> GAMEGFKANLSLLRRPGEKTYTQRCRLFVGNLPADITEDEFKRLFAKYGEPGEVFINKGKGFGFIKLESRALAEIAKAELDDTPMRGRQLRVRFATHAAALSVRNLSPYVSNELLEE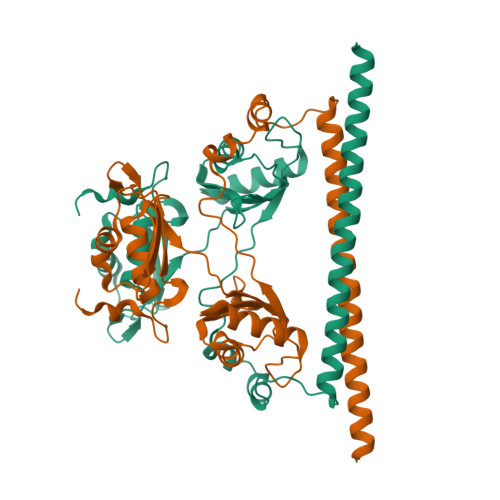AFSQFGPIERAVVIVDDRGRSTGKGIVEFASKPAARKAFERCSEGVFLLTTTPRPVIVEPLEQLDDEDGLPEKLAQKNPMYQKERETPPRFAQHGTFEYEYSQRWKSLDEMEKQQREQVEKNMKDAKDKLESEMEDAYHEHQANLL>GKGTCILVGGHEITSGLEVISSLRAIHGLQVEVCPLNGCDYIVSNRMVVERRSQSEMLNSVNKNKFIEQIQHLQSMFERICVIVEKDREKTGDTSRMFRRTKSYDSLLTTLIGAGIRILFSSCQEETADLLKELSLVEQRKNVGIHVPTVVNSNKSEALQFYLSIPNISYITALNMCHQFSSVKRMANSSLQEISMYAQVTHQKAEEIYRYIHYVFDIQMLPNDLNQDRLKSDI[2x];>[2x]MEKNPPDDTGPVHVPLGHIVANEKWRGSQLAQEMQGKIKLIFEDGLTPDFYLSNRCCILYVTEADLVAGNGYRKRLVRVRNSNNLKGIVVVEKTRMSEQYFPALQKFTVLDLGMVLLPVASQMEASCLVIQLVQEQTKEPSKNPLLGKKRALLLSEPSLLRTVQQIPGVGKVKAPLLLQKFPSIQQLSNASIGELEQVVGQAVAQQIHAFFTQPR

FANCM is crucial in genome maintenance, functioning in the Fanconi anemia (FA) pathway, alternative lengthening of telomeres (ALT), and replication fork protection. FANCM recognizes branched DNA structures and promotes their remodeling through ATP-dependent branch migration. Here we present crystal structures of FANCM’s N-terminal ATP-dependent translocase domain (2.2 Å) and C-terminal FAAP24-bound region (2.4 Å), both complexed with branched DNA. The N-terminal translocase domain specifically recognizes DNA junctions through multiple key elements, while the C-terminal FAAP24-binding domain engages adjacent double-stranded DNA.

To understand how FANCM’s different regions cooperate in DNA recognition, we further determined the crystal structure of its C-terminal region bound to FAAP24 and branched DNA at 2.4 Å resolution. Two copies of the complex are present in the asymmetric unit, related by non-crystallographic symmetry, which bind the duplexes in a head-to-tail arrangement (Fig. EV3A). The splayed arm DNA bases were not visible in the electron density, indicating that they were conformationally disordered and therefore not bound specifically by the protein. In contrast to that structure which showed calcium ions at each FAAP24 (HhH)2 domain-DNA interface and in the FANCM pseudonuclease domain (PND) active site, our new structure showed magnesium ions in the first FAAP24 HhH domain and another in the FAAP24-PND outside the active site (Fig. EV3B). The new structure also reveals a previously unappreciated 5 bp dsDNA binding site within the FANCM pseudonuclease domain complementing the known contact with an additional five base pairs of DNA by FAAP24’s HhH domain. Separated by an eight basepair gap, this arrangement enables recognition of approximately 18 continuous base pairs, substantially more than previously known DNA-binding sites in the complex (Fig. EV3A,B). In striking contrast, removal of FAAP24, which binds FANCM’s C-terminal domain, severely compromised the stimulatory activity (lanes 9–11). An inefficient coupling of ATPase and translocase activity was also seen when FAAP24 was removed from the complex, revealing that FANCM’s C-terminal domains optimize its motor efficiency. A patient-derived mutation truncating the C-terminal HhH domain (p.Arg1931∗; rs144567652) associated with cancer predisposition and infertility showed similar defects, and is consistent with previous observations that both the C-terminal region and FAAP24 are essential for FANCM function.> MKTRKLTNILSKLIDKTMAGTSKITDFTPGSASRSLLEAVSLEIEQFYILTKENIDWGIQEGIIEAFDFQKRQSKRAYGDVTIQFYQPLDMRMYIPAGTTFTSTRQEYPQQFETLVDYYAEPDSTEIVVEVYCKETGVAGNVPEGTINTIASGSSLIRS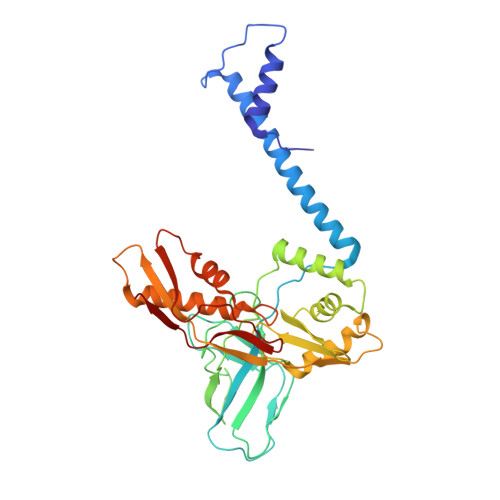VNNEYSFNTGTKEESQEDFKRRFHSFVESRGRATNKSVRYGALQIPDVEGVYVYEETGHITVFAHDRNGNLSDTLKEDIIDALQDYRPSGIMLDVTGVEKEEVNVSATVTISNKSRIGDTLQKHIESVIRSYLNNLKTSDDLIITDLIQAIMNIDDVLIYDVSFDNLDENIIVPPQGIIRAGEIKVELK> VEATAQETDRPRFSFSIAAREGKARTGTIEMKRGVIRTPAFMPVGTAATVKALKPETVRATGADIILGNTYHLMLRPGAERIAKLGGLHSFMGWDRPILTDSGGYQVMSLSSLTKQSEEGVTFKSHLDGSRHMLSPERSIEIQHLLGSDIVMAFDECTPYPATPSRAASSMERSMRWAKRSRDAFDSRKEQAENAALFGIQQGSVFENLRQQSADALAEIGFDGY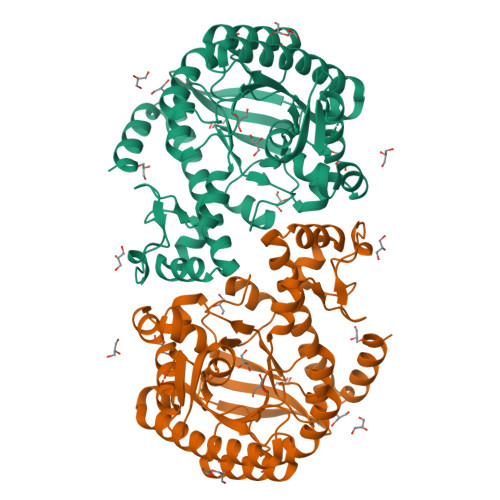AVGGLAVGQGQDEMFRVLDFSVPMLPDDKPHYLMGVGKPDDIVGAVERGIDMFDCVLPTRSGRNGQAFTWDGPINIRNARFSEDLKPLDSECHCAVCQKWSRAYIHHLIRAGEILGAMLMTEHNIAFYQQLMQKIRDSISEGRFSQFAQDFRARYFARNS>[2x]MAPLKLNSRNLSQIAAAGGALVKIPTYQRGRAVKEGIVHIGVGGFHRAHLAVYIDQLMQKHGVNDYAICGVGLQPFDSAMRDALASQDHLYTLIERSAKGSFAHVIGSINSYLFAPDNREAVIAKMAHPDTKIVSLTITESGYYYNENTHELQSEHPDIQFDLDPANEKAPRTTFGFLYAGLTRRYQQGLKPFTVMSCDNMQKNGSITRHMLESFARLRNPEVAEWIAEEGAFPNAMVDRI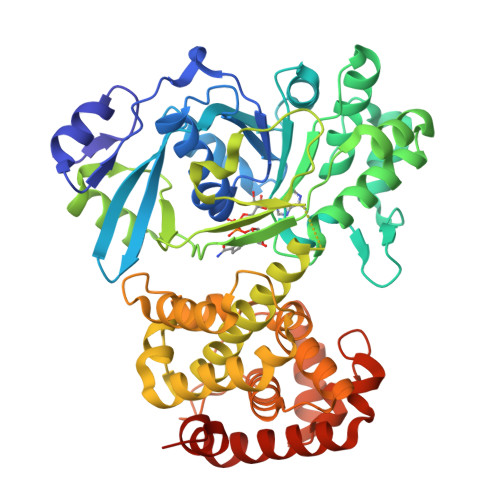TPQTSETDKTALAEKFGIVDSWPVVTEPFTQWVIEDQFSDGRPPFEKVGVQVVKDVHAVEQFEKHKLRLLNGSHSALGYPGQLAGFQYVHEVMANPLFRKFVWQMMQEEVKPLLPEIPGVDIDEYCNTLIERFTNPTIMDQLPRICLNASGKIPQFIMPSIAEAIWETGPFRRLCFVAAAWFHYIKGVDDRGKPFEVVDPMREELQAKARAGGNDPSELLSIKSLFGDDLRNDERFLREITTAMNDIARDGIMKTLPKYINGSHHHHHH> MIGKKILGERYVTVSEAAEIMYNRAQIGELSYEQGCALDYLQKFAKLDKEEAKKLVEELI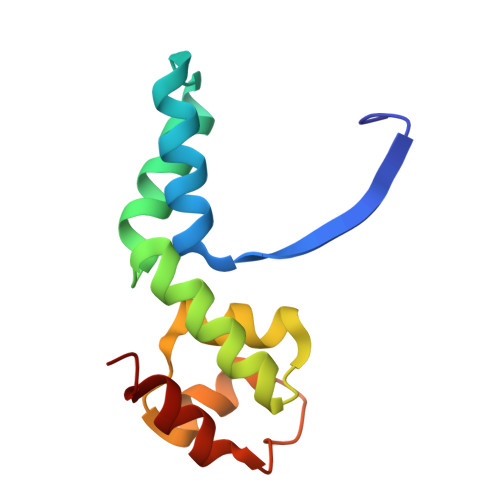SLGIDEKTAVKIADILPEDLDDLRAIYYKRELPENAEEILEIVRKYI> MKNVLMVTTSHDVMGNSNEKTGLWLSELTHPYYSIID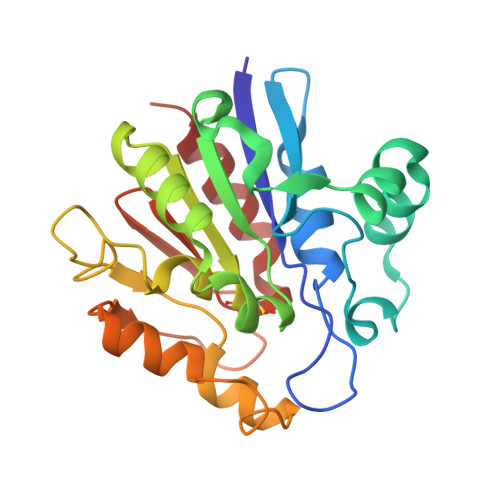KNINIDIVSIMGGEIPIDPNSVAQEDYYNDKFLADDNLKNIMKNSTSLRDVNIKEYDAIIFAGGHGTMWDFPNNANIHSKVLDIYAKNGVIGAICHGVAALINVKDNNGQNIIRDKEVTGFSNNEEKIVGLTDVVPFSLEDSLVEAGAKYSSASEWQSYVKSDSKIITAQNPQSATDFAKAIKQSLFN> HHHHHHHHSQAGDTLNDVIQDPTRRNKL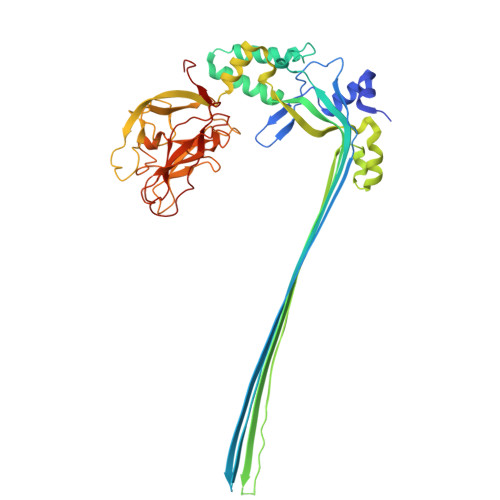INDNNLLKGIIMGRDGPVPSSRELIVRPDTLRAIINNRATIETTTMEAEFTETLMESNYNSASVKVSAPFITANSEYSESSSFKNTETEKSMYTSSRYLFPQGRIDFTTPDSGFDDVIKLSPQFTSGVQAALAKATGTEKREALQNLFQEYGHVFRTKVHIGGVLSAHTMETFSRSENETEVKQDVKAGLEGAVKGWGGGATAGHGNTQGTITTSQNRKLNVKYIVNGGDYTKIQNTEEWVASTNQSEHWRVIEVTEVTAVADLLPQPIRGQVKDLLKPLLGKWVDVEKVPGLESLPVSVYRPKGAIPAGWFWLGDTADASKALLVKPTLPARSGRNPALTSLHQGSGMTEQPFVDLPQYQYLSTYFGSFAHDTPPGSTLRGLRPDHVLPGRYEMHGDTISTAVYVTRPVDVPFPEDECFDLKSLVRVKLPGSGNPPKPRSALKKSMVLFDSGEK>[8x]MSQLAHNLTLSIFDPVANYRAARIICTIGPSTQSVEALKGLIQSGMSVARMNFSHGSHEYHQTTINNVRQAAAELGVNIAIALDTKGPEIRTGQFVGGDAVMERGATCYVTTDPAFADKGTKDKFYIDYQNLS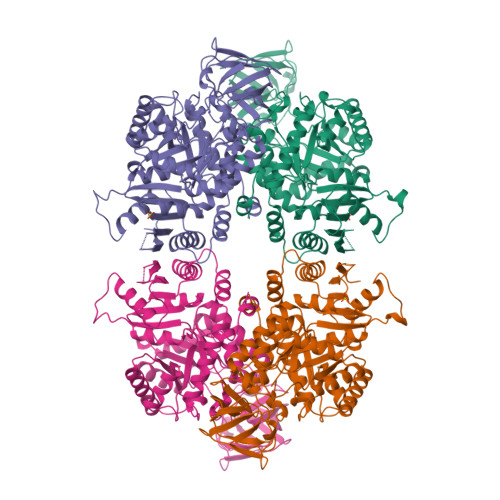KVVRPGNYIYIDDGILILQVQSHEDEQTLECTVTNSHTISDRRGVNLPGCDVDLPAVSAKDRVDLQFGVEQGVDMIFASFIRSAEQVGDVRKALGPKGRDIMIICKIENHQGVQNIDSIIEESDGIMVARGDLGVEIPAEKVVVAQKILISKCNVAGKPVICATQMLESMTYNPRPTRAEVSDVANAVFNGADCVMLSGETAKGKYPNEVVQYMARICLEAQSALNEYVFFNSIKKLQHIPMSADEAVCSSAVNSVYETKAKAMVVLSNTGRSARLVAKYRPNCPIVCVTTRLQTCRQLNITQGVESVFFDADKLGHDEGKEHRVAAGVEFAKSKGYVQTGDYCVVIHADHKVKGYANQTRILLVE>MEPTTEIQATEDLTLSGDHAAASADSLVVDNANDNAGQEEGFEIVLKDDETAPKQDPAKNAEFARRRIERKRQRELEQQMEAVKRGELPESLRVNPDLPPQPDINAYLSEEGLAKYDYDNSRALAAFNAANTEWLMKAQDARSNAVAEQGRKTQEFTQQSAQYVEAARKHYDAAEKLNIPDYQEKEDAFMQLVPPAVGADIMRLFPEKSAALMYHLGANPEKARQLLAMDGQSALIELTRLSERLTLKPRGKQISSAPPADQPITGDVSAANKDAIRKQMDAAASKGDVETYRKLKAKLKGIR[2x]

Tailed double-stranded DNA (dsDNA) bacteriophages and their eukaryotic counterparts, such as herpesviruses, possess a dodecameric portal at a unique vertex of the capsid; this portal serves as a channel for DNA packaging during viral assembly and delivery. The portal interacts with multiple copies of a scaffolding protein (SP) to form a nucleation complex, which initiates the assembly of the major capsid protein (i.e., coat protein) and other minor proteins into a procapsid. The P22 procapsid consists of an icosahedral coat comprising 415 coat protein (gene product [gp] 5) subunits, a dodecameric ring comprising portal protein (gp1) subunits located at a unique capsid vertex, and an internal core comprising approximately 250–300 SP (gp8) subunits and 3 ejection proteins. In this study, we present the structure of the SP gp8 in complex with the dodecameric portal in the P22 procapsid at subnanometer resolution.

Each nodule comprised two copies of the base domain (base dimer) interacting with each other. We referred to the bases near the portal axis as inner base and those far from the axis as outer base. The two base domains likely interacted through electrostatic interactions. Residues Arg240, Glu243, and Arg244 of the inner base domain were located close to residues Arg240 and Glu243 of the outer base domain. Furthermore, each nodule interacted with the portal through the stacking of the inner base on a loop (residues 495–504) of the portal wing. Local reconstruction of the side nodule and stalk-like structure revealed that the side nodule comprised two copies of the base domain, whereas the stalk comprised the column domain, which connected one of the two base domains in the side nodule. The nodules, side nodules, and windmill blades were all dimers of the SP base domain. The SP dimer primarily forms through interactions between two copies of the same α-helix (residues 231–245) within the base domains; this explains why a recombinant SP fragment (residues 238–303) weakly self-associates into dimers.Thosea asigna virus (TaV) is a (+) ssRNA virus that infects the larvae of a defoliating moth (Setothosea asigna) and the prototypic member of the Permutotetraviridae family. In a previous work we have structurally and functionally characterized the non-canonical RdRP domain of TaV (TaVpol: residues 1-674 of the ORF1 product), showing close resemblances with flaviviral RdRPs. In these enzymes, motif C is located upstream of motif A forming a noncanonical C–A–B–D arrangement with a unique connectivity of the major structural elements of the active site. Here we report the X-ray structures of TaVpol captured in three replication-elongation states, revealing high resolution mechanistic details of different events in the nucleotide addition cycle for a non-canonical RdRP.

The X-ray analysis of the Δ10-TaVpol construct, crystallized in the presence of large amounts of Mg2+ (19% PEG 3350, 0.18 M MgSO4), revealed the existence of a second metal ion-binding site located nearby the catalytic cavity, in a non-catalytic position. The resulting electron density maps at 2.07 Å resolution showed strong peaks of extra density in the two molecules of the asymmetric unit. The Mg2+ ions were located at 7 Å from the catalytic aspartate D351 (motif C), coordinated by the side chain carboxyl oxygen of D352 (motif C) and five water molecules, in a perfect octahedral geometry. The solvent molecules participating in Mg2+ coordination appear also to interact with the polymerase side chains of residues of D369: w1, w2 and w3; T353: w4, with the main chain N and carboxyl oxygens of residues T353 (N), P368 (O)M w4, with the main chain oxygen of K51: w3 and with the main chain oxygen of C3676: w5. The presence of non-catalytic Mg2+ ions at the polymerases central cavity were previously described in other RdRPs and recently, the role of these ions in the nucleotide addition cycle has been reviewed by Gong and collaborators. The position of the noncatalytic Mg2+ in Δ10-TaVpol perfectly match that identified in other RdRP structures prior to active site closure.

>MGSSHHHHHHSQDLENLYFQGGSTRLSLEAMLAERAMVARQDLAGLKRKLAGADRVLAPQSPEQCGRESAQAQARSVTSELKSAVKEAQGLEHQTLDFLEQLGEYPVCGILHGDHPVHPSGTHNNNGKVSVKRQFAAGVNTSDALTCAFRFEDSDLVRETALKTTYTDGTWAGFVQRLKMQTTRKCVQEKVSRKLLKQLFPYDPQKLVDVSGELSELVLGIKTNAIASAGPPYWRTKRDALPDMLDCVLPLLYDHIVRKDLTTLRNKHPELFLAECKNKTDRYEVESLGEKTRPYFSHPFHLSALVSVLSQSFSGALKIMTEDSTSFNAYGFSWTNGGAEDLAIWARQAGEAGKKPPRIACYGDDTDIYYRKDGKLYRICPDFKQMDGSVDATTIEAVVDYVVDAHVKQYPTARQFWEEVGKLWVEMATQSPFLIDGTKVYRKMQKDGLMTGVVGTTLFDTVKSALAYNDWADQLMFGSLNLLEEKYAIEFFKNKHGLVIKEGTWKPALVNEDPGFGELWTEQKFLGLQLKVVRRENEKVYVPNLPFEDWLTMWVTPRSKYRSKETETMRERTLFDRARGLLVTGAVFDERARGLMGAVINSTAPEVVCMRVQEGGGRGAPPAYAFLTRDGVFEFPISDGYPSYDWVVSLYSRDHPCDMPRVFPEAATLIASYRKQVMDTRVVI[2x]>[2x]MGSSHHHHHHPAPVEVTYKNMRFLITHNPTNATLNKFIEELKKYGVTTIVRVSEATYDTTLVEKEGIHVLDWPFDAGAPPSNQIVDDWLSLVKIKFREEPGCCIAVHCVAGLGRAPVLVALALIEGGMKYEDAVQFIRQKRRGAFNSKQLLYLEKYRPKMRLRF

pmcPhosphatases of regenerating liver (PRL or PTP4A) are a small family of three cysteine-based phosphatases (also known as PTPs). PRLs employ a two-step catalytic mechanism: (i) formation of a phosphoenzyme intermediate by dephosphorylating substrate and (ii) hydrolysis of the phosphocysteine intermediate and release of free phosphate. The catalytic site is highly conserved and formed by a phosphate-binding loop (P-loop) and a WPD acidic loop. In addition to dephosphorylating substrates, PRLs act as pseudo-phosphatases and bind CBS-pair domain divalent metal cation transport mediators (CNNMs) to regulate magnesium transport.

We use this C49S/D72A double mutant to determine the crystal structure of the cysteine-phosphorylated form of PRL1 (PTP4A1). Small crystals of PRL1 C49S/D72A were obtained with 4′-MUP in the crystallization solution to maintain cysteine phosphorylation. The asymmetric unit contains two PRL1 molecules. PRL1 displays the characteristic cysteine-based phosphatase fold, composed of a five-stranded central β-sheet surrounded by two α-helices on one side and a four-helical bundle on the other side. The omit map clearly shows the density corresponding to the phosphate attached to the catalytic cysteine 104. The positively charged side chain of the catalytic Arg110 interacts electrostatically forming a salt bridge with the negatively charged phosphate group. Hydrogen bonds from backbone amides in the P-loop and an alpha-helix dipole stabilize the position of the phosphate. All three structures show the loop closed with the aspartic acid positioned above the phosphocysteine, ready to initiate hydrolysis. The structure of PRL2 bound to CNNM3 shows an aspartate sidechain inserts into the PRL active site interacting with the arginine in the PRL P-loop. A side-by-side comparison of the structures of the PRL–CNNM complex and the phosphocysteine intermediate shows the phosphate group precludes the CNNM aspartate entering the PRL active site. Mutating the alanine to serine increases phosphocysteine hydrolysis more than 15-fold. In the absence of both aspartic acid and serine/threonine, the phosphocysteine intermediate of PRL1 is stable for weeks.>[2x]MKNLRYKLLLFVFIGFWGLLALNLFILSVKNQEYYEKLAERNMTKKEFLVPTRGNITDRNDEFLATNELVFGVFLPSGLKQKDLLEKIEIIQKFFPNFSKETLLNNYQKENSLY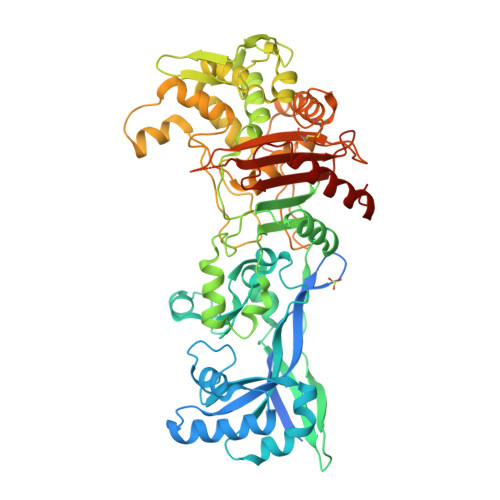NHNLIKVVGFIPYATMQPLYAKLIQTQGIFALPLDKRYYPNNALASHVLGYVGVASLQDLKDDEENQYSQIVGKTGIEKEYNKLLQGKVGYKIMRVNALNQELATLEVVLPSTNNHLQLSLDKRLQKEADKLFENKRGAILVMDAENGELLVAGSYPEYNLNDFVGGISQDKWQKLQDDIYNPLLNRFANALYPPGSVVKMGVGLSFLENLHITENTTIPTPPFIEVGKHKFRDWKKTGHGNSNLYKAIRESVDVYFYKFGLEISIEKLSKTLREVGFGEKTGVDLPNEFVGIVPDNLWKLKRFNQDWRVGDTLITAIGQGSFLATPLQVLAYTGLIATGKLATPHFAINNKQPLKDPLNSFQKKKLQALRVGMYEVCNHKDGTAYHSTRGSKITLACKTGTAQVVEIAQNIVNRMKEKDMEYFHRSHAWITAFLPYEKPKYAITILVEHGEGGSKLGGLLVKMSNKLYELGYLHHHHHH> MSLAADKVDILYLEDDEVDIQSVERVFHKISSLIKIEIAKSGNQALDMLYGRNKENKIHPKLILLDINIPKMNGIEFLKELRDDSSFTDI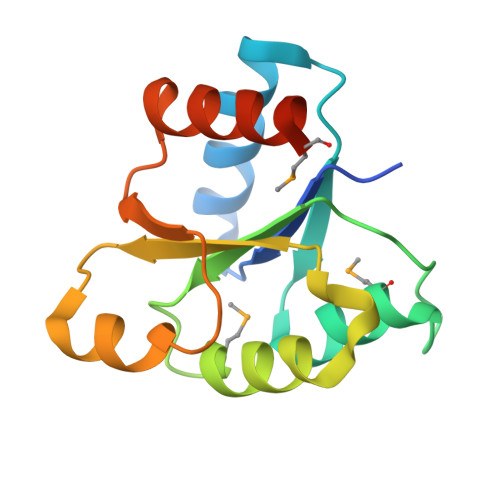EVFVLTAAYTSKDKLAFESLNIRGHLIKPLDYGEAIKLFWILQSMEGHHHHHH> MSVEKIPGYTYGETENRAPFNLEDLKLLKEAVMFTAEDEEYIQKAGEVLEDQVEEILDTWAGFVGSHPHLLYYFTSPDGTPNEKYLAAVRKRFSRWILDTSNRSYDQAWLDYQYEIGLRHHRTKKNQTDNVESVPNIGYRYLVAFIYPITATMKPFLARKGHTPEEVEKMYQAWFK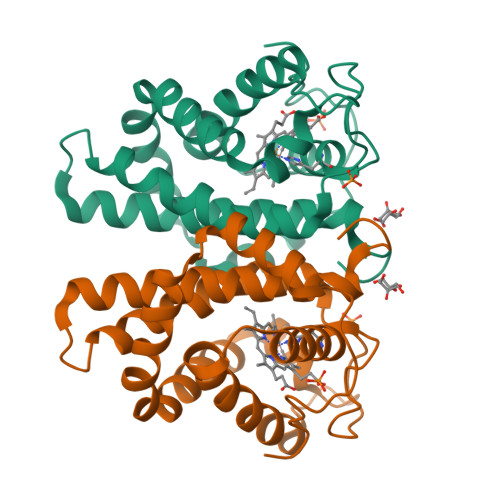ATTLQVALWSYPYVKYGDF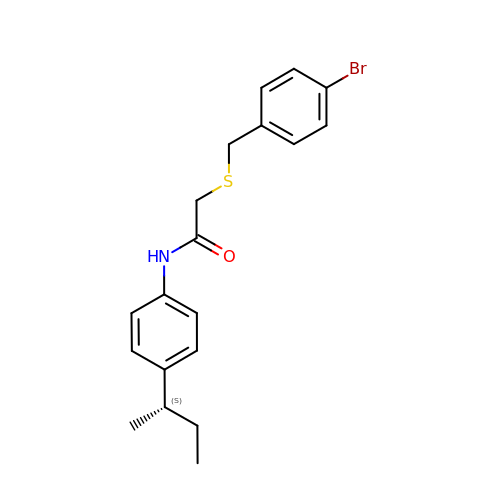2-[(4-bromophenyl)methylsulfanyl]-~{N}-[4-[(2~{S})-butan-2-yl]phenyl]ethanamide | C19 H22 Br N O S | QKUYZJOTWYRWNF-AWEZNQCLSA-N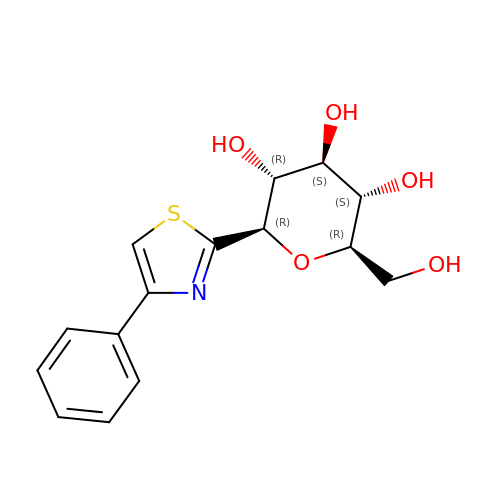(2~{R},3~{S},4~{S},5~{R},6~{R})-2-(hydroxymethyl)-6-(4-phenyl-1,3-thiazol-2-yl)oxane-3,4,5-triol | C15 H17 N O5 S | CQDQZIAPWGJSQJ-RKQHYHRCSA-N> MAHHHHHHMNSLQDLIEQAFENRQNLSLDTASSDLINAINEVLSGLDNGQFRVAEKINGEWTVHQWLKKAVLLSFKLFPNQIIDAGFCKFYDKIPLKYTDCSNEQFQQSGVRVVPHAMVRRGAYIAKNTVLMPSYVNIGAYIDEGVMVDTWATVGSCAQIGKNVHISGGAGIGGV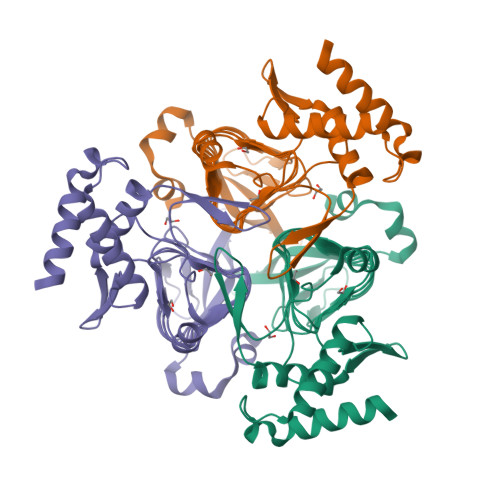LEPLQANPTIIEDNCFIGARSEIVEGVIVEKNSVISMGVFLGQSTKIYNRITGEVSYGRIPAGSVVVAGNLPSHDGSHSLYCAVIVKQVDEKTRAKVSINDLLRANQDD>FSQLLALASLLGQQQAEVQRCREDLQKKESLM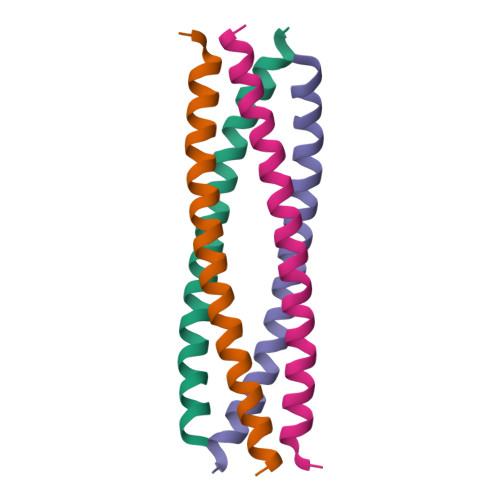METIAKIKALALEHHHHH[2x]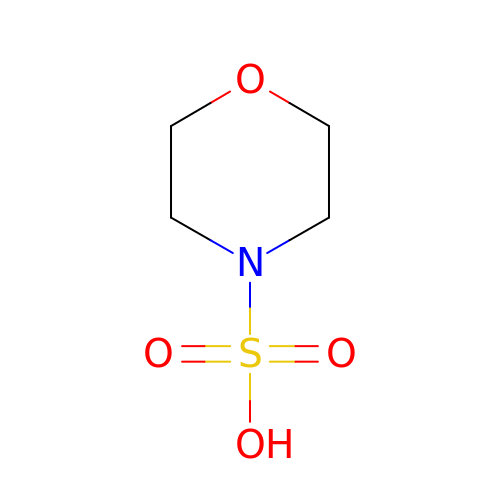morpholine-4-sulfonic acid | C4 H9 N O4 S | GLGNSAPAWZUDRT-UHFFFAOYSA-N> EQGDIVVALYPYDGIHPDDLSFKKGEKMKVLEEHGE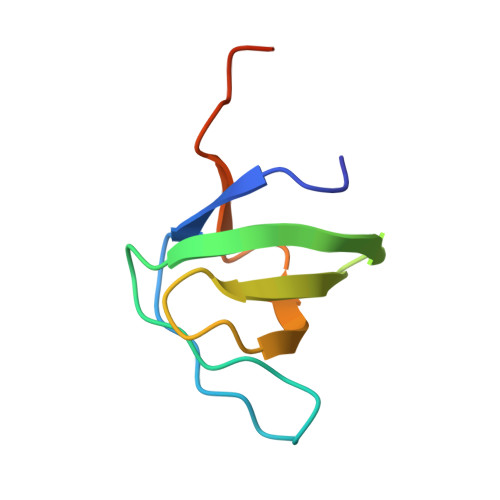WWKAKSLLTKKEGFIPSNYVAKLNTLEHHHHHH> GPKHERFIAYVGIPMLTIQARENDDQIILGSLGSQRMKYIEDENQNYTNISSEYYSQSSMQAVPMYYFNVPKGQWSVDISCEGYQPTSSTSDPHRGRSDGMIAYSNADSDYWNVGEADGVKISKLRNDNTYRQGHPELEINSCHFREGQLLERDATISFHVEAPTDGRFFLVGPAIQKTAKYNYTISYGDWTDRDMELG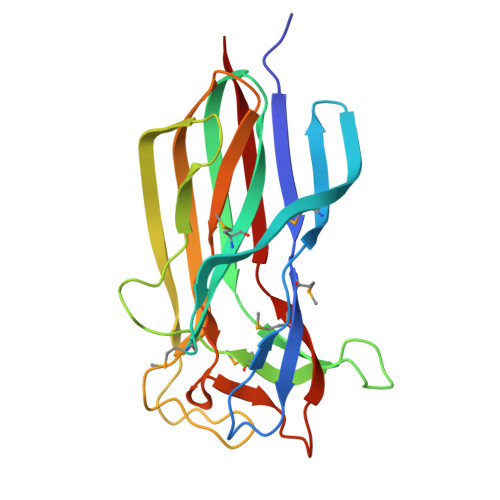LITVVLDEHL>[4x]DQVDVKDC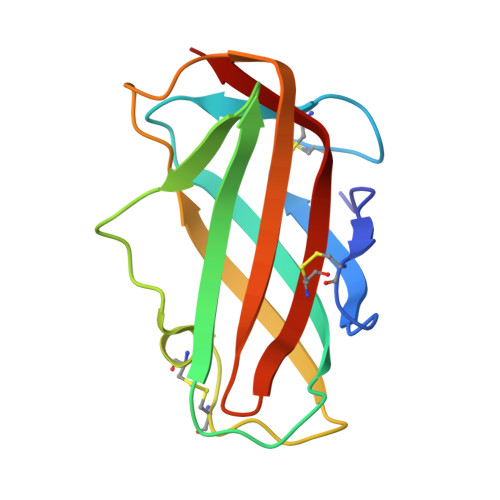ANNEIKKVMVDGCHGSDPCIIHRGKPFTLEALFDANQNTKTAKIEIKASLDGLEIDVPGIDTNACHFVKCPLVKGQQYDIKYTWNVPKIAPKSENVVVTVKLIGDNGVLACAIATHGKIRD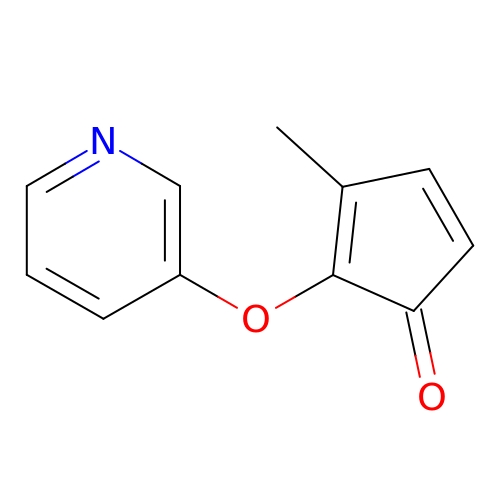3-methyl-2-[(pyridin-3-yl)oxy]cyclopenta-2,4-dien-1-one | C11 H9 N O2 | OXHUSRBHFWQZGQ-UHFFFAOYSA-N> MSQRI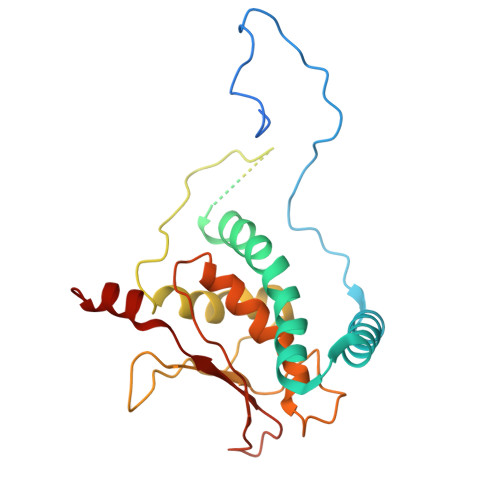IQPSASDQQFPGKSDGYEYTVGPKQAITSEASTTYYISRIYSESLLFKRQEASLSAMAFLFQEMISQLHRTCKTAGDFETKLSDYGHNIGIRLLELLNFRASVSPSSLPRASAFLSQNESSSKLSNASNSPGMLANSSTATSASANERLQEKQTESLSNYITKMRRRDLKILDILQFIHGTLWSYLFNHVSDDLVKSSERDNEYMIVDNFPTLTQFIPGENVSCEYFVCGIIKGFLFNAGFPCGVTAHRMPQGGHSQRTVYLIQFDRQVLDREGLRFG> PNVSRTIARELKSFLLEYTDETGRSVYGARIRTLGEMNSESLEVNYRHLAESKAILALFLAKCPEEMLKIFDLVAMEATELHYPDYARIHSEIHVRISDFPTIYSLRELRESNLSSLVRVTGVVTRRTGVFPQLKYVKFNCLKCGSILGPFFQDSNEEIRISFCTNCKSKGPFRVNGEKTVYRNYQRVTLQEAPGTVPPGRLPRHREVILLADLVDVSKPGEEVEVTGIYKNNYDGNLNAKNGFPVFATIIEANSIKRREGNTANEGEEGLDVFSWTEEEEREFRKISRDRGIIDKIISSMAPSIYGHRDIKTAVACSLFGGVPKNVNGKHSIRGDINVLLLGDPGTAKSQILKYVEKTAHRAVFATGQGASAVGLTASVRKDPITKEWTLEGGALVLADKGVCLIDEFDKMNDQDRTSIHEAMEQQSISISKAGIVTTLQARCSIIAAANPNGGRYNSTLPLAQNVSLTEPILSRFDILCVVRDLVDEEADERLATFVVDSHVRSHPENDEDREGEELKNNGESAIEQGEDEINEQLNARQRRLQRQRKKEEEISPIPQELLMKYIHYARTKIYPKLHQMDMDKVSRVYADLRRESISTGSFPITVRHLESILRIAESFAKMRLSEFVSSYDLDRAIKVVVDSFVDAQKVSVRRQLRRSFAIY;> PDAVFGDRVRRFQEFLDTFTSYRDSVRSIQVYNSNNAANYNDDQDDADERDLLGDDDGDDLEKEKKAASSTSLNILPHRIIISLDDLREFDRSFWSGILVEPAYFIPPAEKALTDLADSMDDVPHPNASAVSSRHPWKLSFKGSFGAHALSPRTLTAQHLNKLVSVEGIVTKTSLVRPKLIRSVHYAAKTGRFHYRDYTDATTTLTTRIPTPAIYPTEDTEGNKLTTEYGYSTFIDHQRITVQEMPEMAPAGQLPRSIDVILDDDLVDKTKPGDRVNVVGVFKSLGAGGMNQSNSNTLIGFKTLILGNTVYPLHARSTGVAARQMLTDFDIRNINKLSKKKDIFDILSQSLAPSIYGHDHIKKAILLMLMGGVEKNLENGSHLRGDINILMVGDPSTAKSQLLRFVLNTASLAIATTGRGSSGVGLTAAVTTDRETGERRLEAGAMVLADRGVVCIDEFDKMTDVDRVAIHEVMEQQTVTIAKAGIHTTLNARCSVIAAANPVFGQYDVNRDPHQNIALPDSLLSRFDLLFVVTDDINEIRDRSISEHVLRTHRYLPPGYLEGEPVRERLNLSLAVGEDADINPEEHSNSGAGVENEGEDDEDHVFEKFNPLLQAGAKLAKNKGNYNGTEIPKLVTIPFLRKYVQYAKERVIPQLTQEAINVIVKNYTDLRNDDNTKKSPITARTLETLIRLATAHAKVRLSKTVNKVDAKVAANLLRFALL;> LRIIWGTNVSIQECTTNFRNFLMSFKYKFRKILDEREEFINNTTDEELYYIKQLNEMRELGTSNLNLDARNLLAYKQTEDLYHQLLNYPQEVISIMDQTIKDCMVSLIVDNNLDYDLDEIETKFYKVRPYNVGSCKGMRELNPNDIDKLINLKGLVLRSTPVIPDMKVAFFKCNVCDHTMAVEIDRGVIQEPARCERIDCNEPNSMSLIHNRCSFADKQVIKLQETPDFVPDGQTPHSISLCVYDELVDSCRAGDRIEVTGTFRSIPIRANSRQRVLKSLYKTYVDVVHVKKVSDKRLDVDTSTIEQELMQNKVDHNEVEEVRQITDQDLAKIREVAAREDLYSLLARSIAPSIYELEDVKKGILLQLFGGTNKTFTKGGRYRGDINILLCGDPSTSKSQILQYVHKITPRGVYTSGKGSSAVGLTAYITRDVDTKQLVLESGALVLSDGGVCCIDEFDKMSDSTRSVLHEVMEQQTISIAKAGIITTLNARSSILASANPIGSRYNPNLPVTENIDLPPPLLSRFDLVYLVLDKVDEKNDRELAKHLTNLYLEDKPEHISQDDVLPVEFLTMYISYAKEHIHPIITEAAKTELVRAYVGMRKMGDDSRSDEKRITATTRQLESMIRLAEAHAKMKLKNVVELEDVQEAVRLIRSAIKDYATDPKTGKIDMNLVQTGKSVIQRKLQEDLSREIMNVLKDQASDSMSFNELIKQINEHSQDRVESSDIQEALSRLQQEDKVIVLGEGVRRSVRL;> NTEIIKSFKNFILEFRLDSQFIYRDQLRNNILVKNYSLTVNMEHLIGYNEDIYKKLSDEPSDIIPLFETAITQVAKRISILSRAQSANNNDKDPENTSMDTDSLLLNSLPTFQLILNSNANQIPLRDLDSEHVSKIVRLSGIIISTSVLSSRATYLSIMCRNCRHTTSITINNFNSITGNTVSLPRSCLSTIESESSMANESNIGDESTKKNCGPDPYIIIHESSKFIDQQFLKLQEIPELVPVGEMPRNLTMTCDRYLTNKVIPGTRVTIVGIYSIYNSKNGAGSGRSGGGNGGSGVAIRTPYIKILGIQSDVETSSIWNSVTMFTEEEEEEFLQLSRNPKLYEILTNSIAPSIFGNEDIKKAIVCLLMGGSKKILPDGMRLRGDINVLLLGDPGTAKSQLLKFVEKVSPIAVYTSGKGSSAAGLTASVQRDPMTREFYLEGGAMVLADGGVVCIDEFDKMRDEDRVAIHEAMEQQTISIAKAGITTVLNSRTSVLAAANPIYGRYDDLKSPGDNIDFQTTILSRFDMIFIVKDDHNEERDISIANHVINIHTGNANAMQNQQEENGSEISIEKMKRYITYCRLKCAPRLSPQAAEKLSSNFVTIRKQLLINELESTERSSIPITIRQLEAIIRITESLAKLELSPIAQERHVDEAIRLFQASTMDAAS;> VDDVTGEKVREAFEQFLEDFSVQSTDTGEVEKVYRAQIEFMKIYDLNTIYIDYQHLSMRENGALAMAISEQYYRFLPFLQKGLRRVVRKYAPXXXXXXXXXXXXXXERVFQISFFNLPTVHRIRDIRSEKIGSLLSISGTVTRTSEVRPELYKASFTCDMCRAIVDNVEQSFKYTEPTFCPNPSCENRAFWTLNVTRSRFLDWQKVRIQENANEIPTGSMPRTLDVILRGDSVERAKPGDRCKFTGVEIVVPDVTQLGLPGVKPSSTLDTRGISKTTEGLNSGVTGLRSLGVRDLTYKISFLACHVISIGXXXXXXXXXXXXXXXXXXXXXXXXXXSDEINELKEMVKDEHIYDKLVRSIAPAVFGHEAVKKGILLQMLGGVHKSTVEGIKLRGDINICVVGDPSTSKSQFLKYVVGFAPRSVYTSGKASSAAGLTAAVVRDEEGGDYTIEAGALMLADNGICCIDEFDKMDISDQVAIHEAMEQQTISIAKAGIHATLNARTSILAAANPVGGRYNRKLSLRGNLNMTAPIMSRFDLFFVILDDCNEKIDTELASHIVDLHMKRDEAIEPPFSAEQLRRYIKYARTFKPILTKEARSYLVEKYKELRKDDAQGFSRSSYRITVRQLESMIRLSEAIARANCVDEITPSFIAEAYDLLRQSIIRVDV;> MSAALPSIQLPVDYNNLFNEITDFLVTFKQDTLSSDATRNENEDENLDAENIEQHLLEKGPKYMAMLQKVANRELNSVIIDLDDILQYQNEKFLQGTQADDLVSAIQQNANHFTELFCRAIDNNMPLPTKEIDYKDDVLDVILNQRRLRNERMLSDRTNEIRSENLMDTTMDPPSSMNDALREVVEDETELFPPNLTRRYFLYFKPLSQNCARRYRKKAISSKPLSVRQIKGDFLGQLITVRGIITRVSDVKPAVEVIAYTCDQCGYEV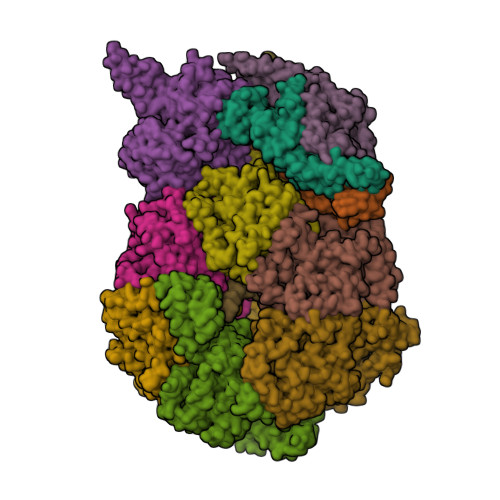FQEVNSRTFTPLSECTSEECSQNQTKGQLFMSTRASKFSAFQECKIQELSQQVPVGHIPRSLNIHVNGTLVRSLSPGDIVDVTGIFLPAPYTGFKALKAGLLTETYLEAQFVRQHKKKFASFSLTSDVEERVMELITSGDVYNRLAKSIAPEIYGNLDVKKALLLLLVGGVDKRVGDGMKIRGDINVCLMGDPGVAKSQLLKAICKISPRGVYTTGKGSSGVGLTAAVMKDPVTDEMILEGGALVLADNGICCIDEFDKMDESDRTAIHEVMEQQTISISKAGINTTLNARTSILAAANPLYGRYNPRLSPLDNINLPAALLSRFDILFLMLDIPSRDDDEKLAEHVTYVHMHNKQPDLDFTPVEPSKMREYIAYAKTKRPVMSEAVNDYVVQAYIRLRQDSKREMDSKFSFGQATPRTLLGIIRLSQALAKLRLADMVDIDDVEEALRLVRVSKESLYQ;> MYGDLGNKLVLEAKRTKQLYARSNQDVNLPMYHEDIIRNILKEVSNLRKNTEYLKEQQQLGMLDDKVAKCQYFVTLLCMERNKRCLLAYQRLRTDILDSMAWNNNGLDLMSSITFSQQDTNNLSHQEQEYLKEYCDLITDLKSGDLVDIDLSGSLVPPSDVFIDVRVLKDAGEIQTEYGVFNLIKDSQFFVRQSDVERLIQQGYLQKI;> LPAHLQQTFSPEEIQFIVENEPIKIFPRITTRQKIRGDDRGTGNHTRWQLITTDDKALNNMVAMRSTEVVLWIALLLKQQSKCSIVAPQWLTTKELDRKIQYEKTHPDRFSELPWNWLVLARILFNKAKDDFHDPIHELRGKIQDLREIRQIKVLKGLKYLNESHLQLDNLSLLEINELRPFITEIMDKLREIHTASL;> YYDIDDVLADGTEFPCKFQYDIPGLGYLENNPGRPITKNTKLSLPLWLARILAIVGGDEALVDEEPVPFVELLPPDMFSTKVMNAIKTDPVALDLHSINSHFFSLAIKWIMLFSEKELANVVSELLLQRAQELNHHASSLSIDLNADSTGKNSANTNIATSTFLLKLEEMEKEIYKKSHESYKDTKRWMFK;> INIDDILAELDKETTAVDSTKITQGSSSTTHRDANTIVGSSLDLNDKTQIYVSPQQDFSDLMKSWKNERCSPELLPYPHQLMKRLLNRISMQSQLIENISMGFLDMQNASNANPPMPNESKLPLLCMETELERLKFVIRSYIRCRLSKIDKFSLYLRQLNEDENSLISLTDLLSKDEIKYHDTHSLIWLKLVNDSILKYMPEELQAINDTEGSVNMIDEPDWNKFVFIHVNGPPDGKWNEDPLLQENEFGKPCYTVTIPDLKEEVELTIGSIYVMRYEVIRDLLRDDKVAL;> ISQFSEAYNKILRNSSSHSSCQLVIFVSCLNIDALCATKMLSLLFKKQLVQSQIVPIFGYSELRRHYSQLDDNINSLLLVGFGGVIDLEAFLEIDPQEYVIDTDEKSGEQSFRRDIYVLDAHRPWNLDNIFGSQIIQCFDDGTVDDTLGEQKEAYYKLLELDEESGDDELSGDENDNNGGDDEATDADEVTDEDEEDEDETISNKRGNSSIGPNDLSKRKQRKKQIHEYEGVLEEYYSQGTTVVNSISAQIYSLLSAIGETNLSNLWLNILGTTSLDIAYAQVYNRLYPLLQDEVKRLTPSSRNSVKTPDTLTLNIQPDYYLFLLRHSSLYDSFYYSNYVNAKLSLWNENGKKRLHKMFARMGIPLSTAQETWLYMDHSIKRELGIIFDKNLDRYGLQDIIRDGFVRTLGYRGSISASEFVEALTALLEVGNSTDKDSVKINNDNNDDTDGEEEEDNSAQKLTNLRKRWVSNFWLSWDALDDRKVELLNRGIQLAQDLQRAIFNTGVAILEKKLIKHLRIYRLCVLQDGPDLDLYRNPLTLLRLGNWLIECCAESEDKQLLPMVLASIDENTDTYLVAGLTPRYPRGLDTIHTKKPILNNFSMAFQQITAETDAKVRIDNFESSIIEIRREDLSPFLEKLTLSGLL> MAGETDLQKILRESNDQFTAQMFSEVVKANPGQNVVLSAFSVLPPLGQLALASVGESHDELLRALALPNDNVTKDVFADLNRGVR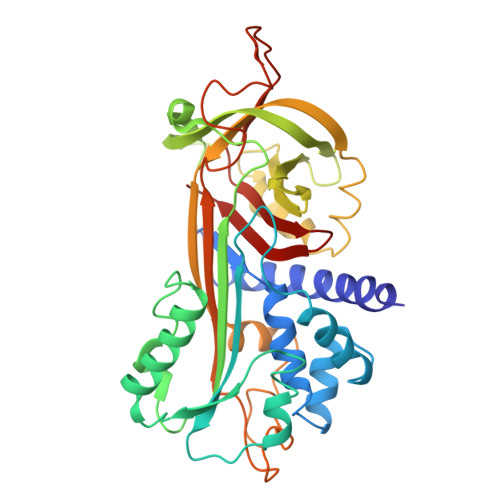AVKGVDLKMASKIYVAKGLELNDDFAAVSRDVFGSEVQNVDFVKSVEAAGAINKWVEDQTNNRIKNLVDPDALDETTRSVLVNAIYFKGSWKDKFVKERTMDRDFHVSKDKTIKVPTMIGKKDVRYADVPELDAKMIEMSYEGDQASMIIILPNQVDGITALEQKLKDPKALSRAEERLYNTEVEITLPKFKIETTTDLKEVLSNMNIKKLFTPGAARLENLLKTKESLTVDAAIQKAFIEVNEEGAEAAAANAFGIVPKSLILYPEVHIDRPFYFELKIDGIPMFNGKVIEP1-amino-9,10-dioxo-4-[(4-sulfamoylphenyl)amino]-9,10-dihydroanthracene-2-sulfonic 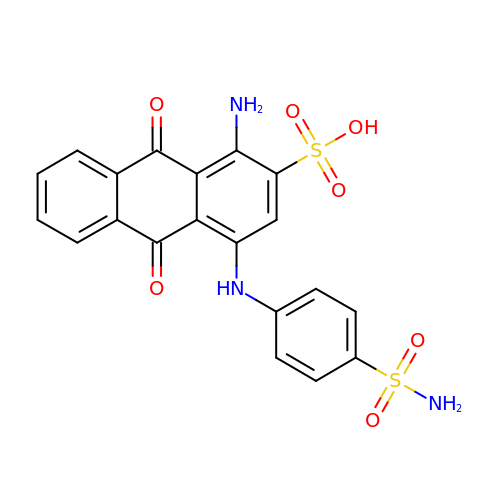acid | C20 H15 N3 O7 S2 | RRARWTAYDLOASH-UHFFFAOYSA-N>[4x]GPGSMARNKIALIGSGMIGGTLAHLAGLKELGDVVLFDIAEGTPQGKGLDIAESSPVDGFDAKFTGANDYAAIEGADVVIVTAGVPRKPGMSRDDLLGINLKVMEQVGAGIKKYAPEAFVICITNPLDAMVWALQKFSGLPAHKVVGMAGVLDSARFRYFLSEEFNVSVEDVTVFVLGGHGDSMVP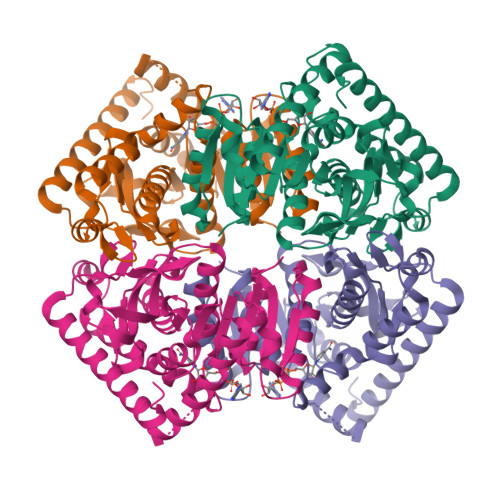LARYSTVAGIPLPDLVKMGWTSQDKLDKIIQRTRDGGAEIVGLLKTGSAFYAPAASAIQMAESYLKDKKRVLPVAAQLSGQYGVKDMYVGVPTVIGANGVERIIEIDLDKDEKAQFDKSVASVAGLCEACIGIAPSLK> PELPEVETVRRELEKRIVGQKIISIEATYPRMVLTGFEQLKKELTGKTIQGISRRGKYLIFEIGDDFRLISHLR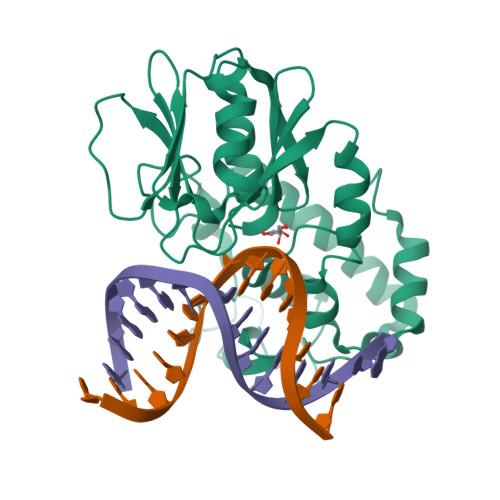MEGKYRLATLDAPREKHDHLTMKFADGQLIYADVRKFGTWELISTDQVLPYFLKKKIGPEPTYEDFDEKLFREKLRKSTKKIKPYLLEQTLVAGLGNIYVDEVLWLAKIHPEKETNQLIESSIHLLHDSIIEILQKAIKLGGSSIRTYSALGSTGKMQNELQVYGKTGEKCSGCGAEIQKIKVAGRGTHFCPVCQQK Here, we present a high-resolution application of SPA to electron crystallography data, using cryo-EM movies of the prokaryotic, cyclic-nucleotide modulated potassium channel MloK1. Each of the four MloK1 monomers forming the pore has a transmembrane domain (TMD), a voltage sensor domain (VSD), and a soluble cyclic-nucleotide binding domain (CNBD), which lies in the intracellular side. The total molecular weight of the tetramer is 160 kDa. Furthermore, we identified different conformations of MloK1 tetramers within the disordered 2D crystals by means of single-particle classification.

We then applied maximum-likelihood 3D classification in FREALIGN28 to determine conformational variations within the 2D crystals, while imposing C4 symmetry and keeping the alignment parameters for the particles constant. To obtain more insight, the consensus atomic model was flexibly fit into each map of the 3D classes using Normal Mode Analysis and then refined in real space. Compared to model #1, the C-terminal helix in “extended”-like model #3 is rotated by about 4 degrees clockwise when seen from the CNBD side, while in the “compact” model #5 it is rotated by about 3 degrees counter-clockwise. A rotation of the selectivity filter by about the same magnitude also occurs in this trajectory. Finally, the most extended conformers of our ensemble (models #1 and #3) also have the S6 helix crossing bundle and the selectivity filter slightly more constricted (<1 Å) than the most compact ensemble members (models #4, #5, and #6). The eight obtained 3D classes have a slightly lower resolution than the consensus map, likely due to the limited number of particles in each class.

>MSVLPFLRIYAPLNAVLAAPGLLAVAALTIPDMSGRSRLALAALLAVIWGAYLLQLAATLLKRRAGVVRDRTPKIAIDVLAVLVPLAAFLLDGSPDWSLYCAVWLLKPLRDSTFFPVLGRVLANEARNLIGVTTLFGVVLFAVALAAYVIERDIQPEKFGSIPQAMWWAVVTLSTTGYGDTIPQSFAGRVLAGAVMMSGIGIFGLWAGILATGFYQEVRRGDFVRNWQLVAAVPLFQKLGPAVLVEIVRALRARTVPAGAVICRIGEPGDRMFFVVEGSVSVATPNPVELGPGAFFGEMALISGEPRSATVSAATTVSLLSLHSADFQMLCSSSPEIAEIFRKTALERRGAAASA[4x]> 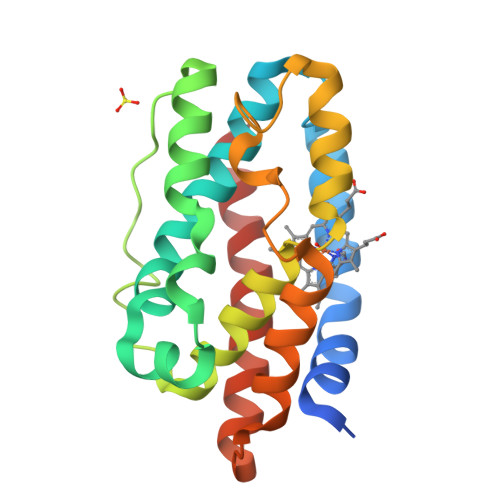MDTLAPESTRQNLRSQRLNLLTNEPHQRLESLVKSKEPFASRDNFARFVAAQYLFQHDLEPLYRNEALARLFPGLASRARDDAARADLADLGHPVPEGDQSVREADLSLAEALGWLFVSEGSKLGAAFLFKKAAALELDENFGARHLAEPEGGRAQGWKSFVAILDGIELNEEEERLAAKGASDAFNRFGDLLERTFA(2R,3S,5S,6R)-5-amino-3-hydroxy-6-methyl-oxan-2-yl | C16 H26 N6 O13 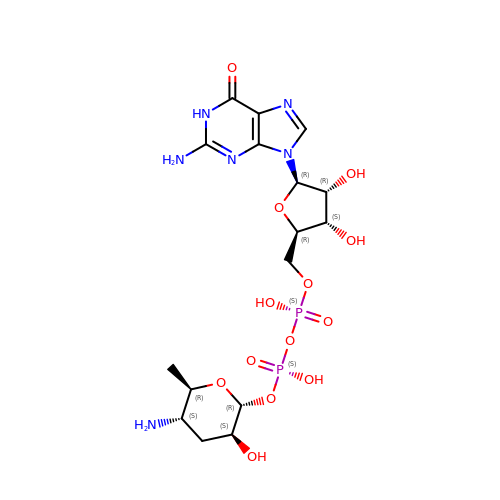P2 | DRNSMVBRYJDNAT-CYCRINRGSA-N>[5x]FTGLTDNLRIGSFGNEVVIELRCAWREGVLLEIMDVISDLHLD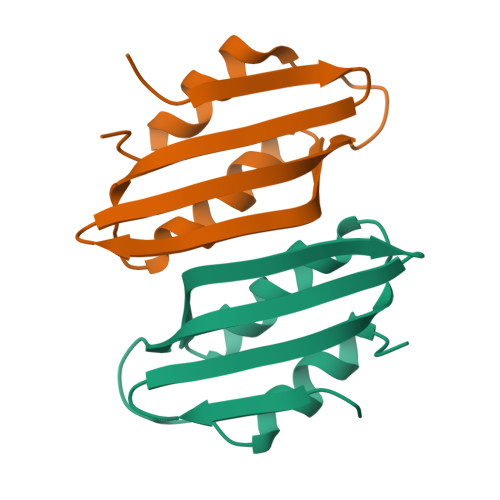SHSVQSSTGDGLLCLTVNCKHKGSKIATPGMIKEALQRVAWIC>APDSVDYRKKGYVTPVKNQGQCGSCWAFSSVGALEGQLKKKTGKLLNLSPQNLVDCVSENDGCGGGYMTNAFQYVQKNRGIDSEDAYPYVGQEESCMYNPTGKAAKCRGYREIPEGNEKALKRAVARVGPVSVAIDASLTSFQFYSKGVYYDESCNSDNLNHAVLAVGYGIQ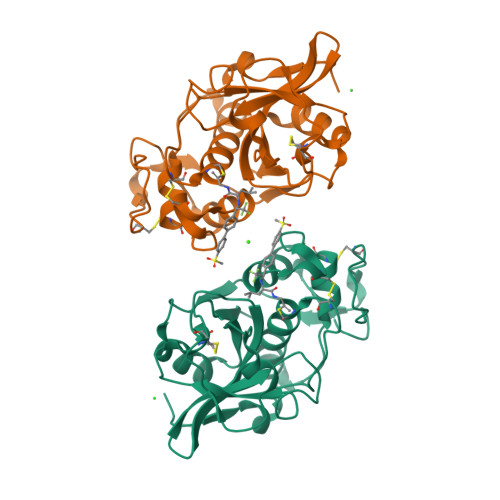KGNKHWIIKNSWGENWGNKGYILMARNKNNACGIANLASFPKM[2x]>MADVVTEFGALTDYRKGGVEIIDDDPRNYVFSNVFEVAANAAPYERVAVGKN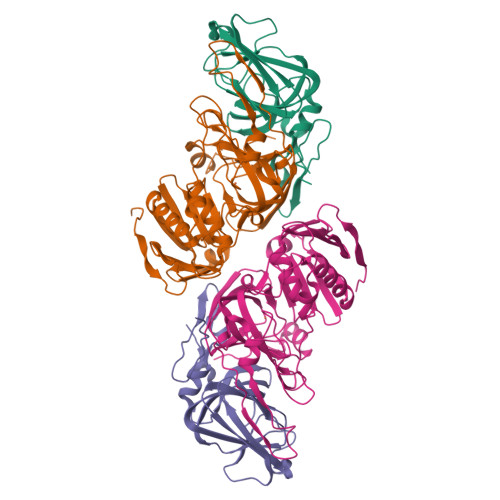FEYVIESARAEGTSGWFSCAHDEFVLAMDGQIEVHLLKLDNSDAYVDPDSEGAVAIGEALPEGRKMGRIVLRRGHMALLPVGAAYRFYAEQPAAMLFQSIEGAVTVQKWGEICQTEAA[4x];>[4x]MAMSEALEIIDFGDSKARTDTEHLAINNETGYRSFRAGGFTFTRDEYFARLTWPGGSHIIPIDAFLRAMMRDVAWGFFYGVVNFDHVFGTINHYGEVTMFAGRFNDAYRNAGRDHEERFKSSALMAVFKDILSDWTVEGYDPFAAPMETGLPWGIKNGNNDEAISRQRVTARRMVGLPGDTPVRTDANGFPVNRQFADVPQEQPVVEAEPGFEAEVSAYNLFGYLSRSDVTWNPSVCSVVGDSLFCPTSEEFILPVEHGNDRCEWFLQLSDEIVWDVKDKESGKPRARVTARAGDICCMPADIRHQGYSTKRSMLLVWENGSPKIPQMIADGTAPVVPVTF1-[(4S)-imidazo[1,2-a]pyridin-7-yl]methanamine 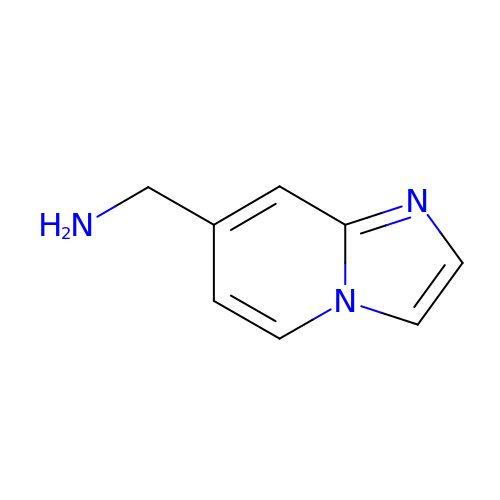| C8 H9 N3 | JOQDUOWWWPMEHJ-UHFFFAOYSA-N>MGSIGEPNRLLCFSIYVTKKPDQSEEDHHNHVSKVNAPMMIPFLKKYGIVRYTVKHNDAYSKPKQAALMAGQPEENVLAYDTVFEMIVKDIESIQTMQKDEEFLRTAIPDLFNFADMTRTKGSGTWIEE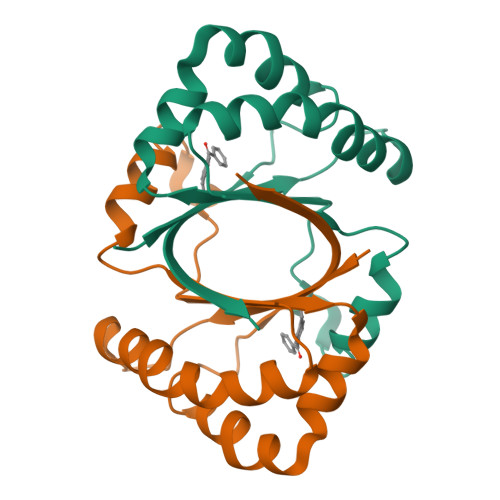FTFALEHHHHHH[2x]> GDPIADMIDQTVNNQVNRSLTALQVLPTAANTEASSHRLGTGVVPALQAAETGASSNASDKNLIETRCVLNHHSTQETAIGNFFSRAGLVSIITMPTMGTQNTDGYANWDIDLMGYAQLRRKCELFTYMRFDAEFTFVVAKPNGELVPQLLQYMYVPPGAPKPTSRDSFAWQTATNPSVFVKMTDPPAQVSVPFMSPASAYQWFYDGYPT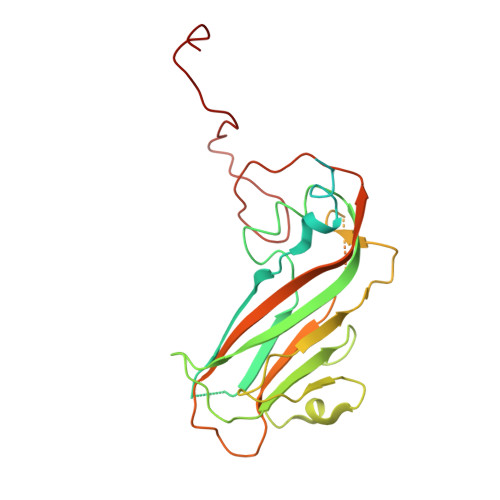FGEHLQANDLDYGQCPNNMMGTFSIRTVGTKKSPHSITLRVYMRIKHVRAWIPRPLRNQPYLFKTNPNYKGNDIKCTSTSRDKITTL>MTGMSREEVESLIQEVLEVYPEKARKDRNKHLAVNDPAVTQSKKCIISNKKSQPGLMTIRGCAYAGSKGVVWGPIKDMIHISHGPVGCGQYSRAGRRNYYIGTTGVNAFVTMNFTSDFQEKDIVFGGDKKLAKLIDEVETLFPLNKGISVQSECPIGLIGDDIESVSKVKGAELSKTIVPVRCEGFRGVSQSLGHHIANDAVRDWVLGKRDEDTTFASTPYDVAIIGDYNIGGDAWSSRILLEEMGLRCVAQWSGDGSISEIELTPKVKLNLVHCYRSMNYISRHMEEKYGIPWMEYNFFGPTKTIESLRAIAAKFDESIQKKCEEVIAKYKPEWEAVVAKYRPRLEGKRVMLYIGGLRPRHVIGAYEDLGMEVVGTGYEFAHNDDYDRTMKEMGDSTLLYDDVTGYEFEEFVKRIKPDLIGSGIKEKFIFQKMGIPFREMHSWDYSGPYHGFDGFAIFARDMDMTLNNPCWKKLQAPWEASEGAEKVAASA[2x];>MSQQVDKIKASYPLFLDQDYKDMLAKKRDGFEEKYPQDKIDEVFQWTTTKEYQELNFQREALTVNPAKACQPLGAVLCALGFEKTMPYVHGSQGCVAYFRSYFNRHFREPVSCVSDSMTEDAAVFGGQQNMKDGLQNCKATYKPDMIAVSTTCMAEVIGDDLNAFINNSKKEGFIPDEFPVPFAHTPAFVGSHVTGWDNMFEGIARYFTLKSMDDKVVGSNKKIN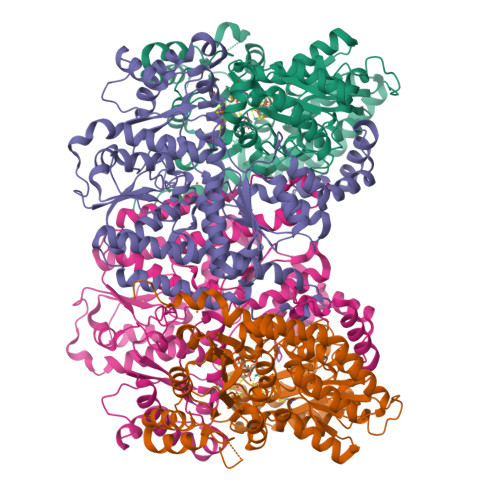IVPGFETYLGNFRVIKRMLSEMGVGYSLLSDPEEVLDTPADGQFRMYAGGTTQEEMKDAPNALNTVLLQPWHLEKTKKFVEGTWKHEVPKLNIPMGLDWTDEFLMKVSEISGQPIPASLTKERGRLVDMMTDSHTWLHGKRFALWGDPDFVMGLVKFLLELGCEPVHILCHNGNKRWKKAVDAILAASPYGKNATVYIGKDLWHLRSLVFTDKPDFMIGNSYGKFIQRDTLHKGKEFEVPLIRIGFPIFDRHHLHRSTTLGYEGAMQILTTLVNSILERLDEETRGMQATDYNHDLVR[2x]>MSYNYLKAARKIICIGRNYAAHIKELNNSTPKQPFFFLKPTSSIVTPLSSSLVKTTRPANSTFNGLNEDGTNPGPIFIPRGVKVHHEIELALIVSKHLSNVTKMKPEEVYDSISGVALALDLTARNVQDEAKKKGLPWTISKGFDTFMPISAIVSREKFSSYKSNLQD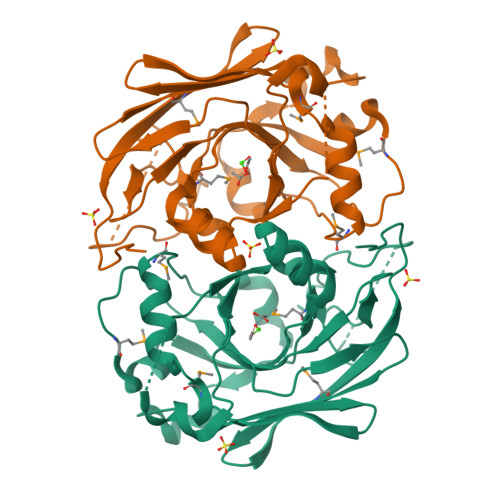IFRVKCSVNGQLRQDGGTNLMLHPLHKILQHISTMISLEPGDIILTGTPAGVGELKPGDRVHCELLQNNDNIVDMNFECENRPGPYEFRET[6x]> GPGS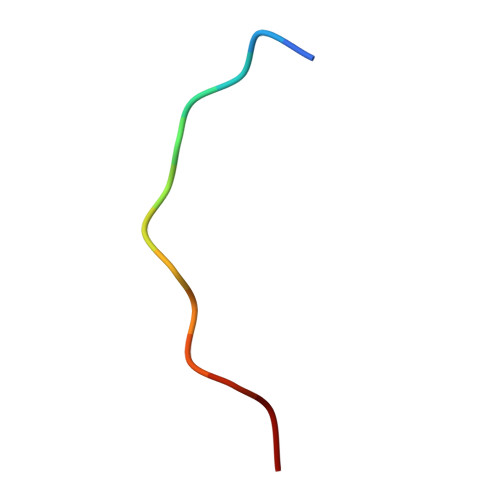EPPPKPPRS>[8x]MPKIILPNFRADYSEQVRDWLGISDATASSTDTTARFLWHAEDGDVLVIPDTVDPDFPGYVADTLGIDGTSVHVERTQTPLSEAVLQDPEFIDRLAAHTGTGAGWSLFPCVSTRAAAQLTRKLNVAALDGYEFAMQNGIDLLNMKSTFRRLAAGLGTPLTDGVVARGPAEVRSAIQELIAETGMVIAKQDRSGGGHGNIGISTSPESSFPGTREVLAYANDQLDTLADTLWSQLTDTQNQFITVETY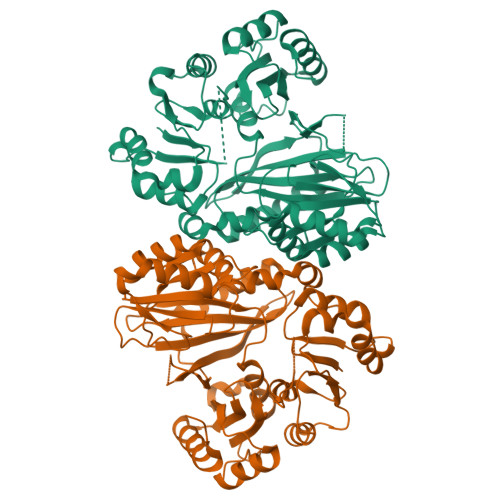HRADQRFFFEYHLDGDRARFLHSSILKYEQLPEGSGGSAKWIGLDSPSRSEFEATLKPAEEFIEMIRTIGYRGYVNIDGIVLDDGRVFFHEINARWSGGLIYHTVAERLLGHDYARNNFFSSILNVVPAGLADLLRSLERAGVRYDKDSGEGAVVLGCNSDLGPGAELLVFSKDWDRLTAMKDEIATTAGTLSLEHHHHHH2-((3',5'-DIMETHOXY-4'-HYDROXYPHENYL)AZO)BENZOIC ACID | 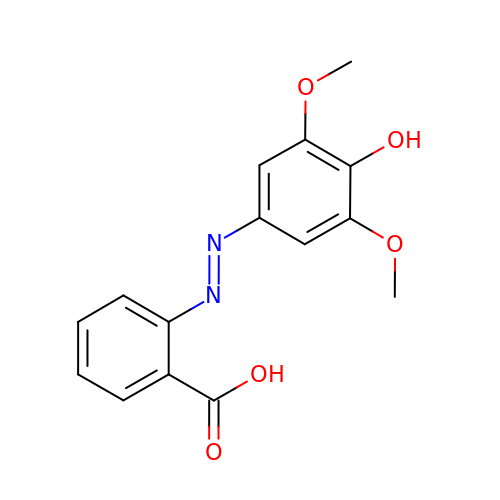C15 H14 N2 O5 | OUUSCQGLQHBVJX-WUKNDPDISA-N> HHHHHHENLYFQGD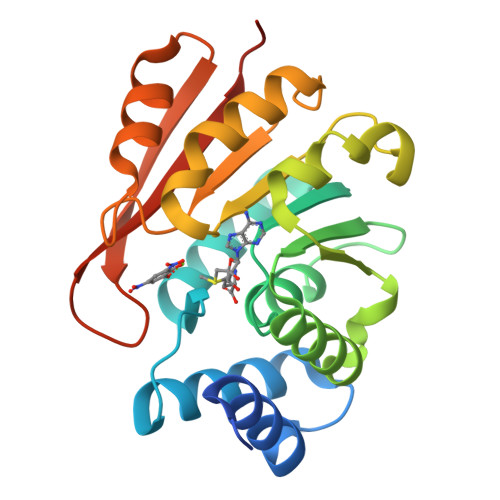TKEQRILNHVLQHAEPGNAQSVLEAIDTYCEQKEWAMNVGDKKGKIVDAVIQEHQPSVLLELGAYCGYSAVRMARLLSPGARLITIEINPDCAAITQRMVDFAGVKDKVTLVVGASQDIIPQLKKKYDVDTLDMVFLDHWKDRYLPDTLLLEECGLLRKGTVLLADNVICPGAPDFLAHVRGSSCFECTHYQSFLEYREVVDGLEKAIYKGPGSEAGP> MKLIGIKTSNCFLVSDNIEGKRYFHSQLDELLFDGKRATETYKSDWFKLEKEPSVIEKQMPAKKINHRYELKEGFQESELTPKVIKASYIGEDSEYYEVKGLYDLKFEEIP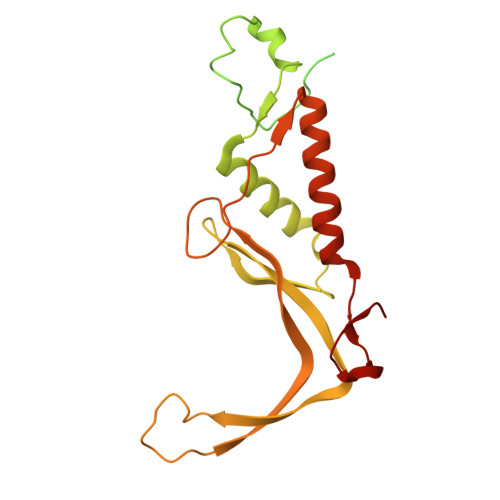QQNEKIEFEMNVIEEIDGELKLQSHNFNLNYNLLDRIQTHPMLLETKPCYLSQEESYKIIRNHIKANINPKFARITSDYDFCLTVVKVLELYKPHEYIVDLNAMYKRRKPKLEKRFQTKREVEIYKVAPKAYQSYPIVEPFSGKDVEDLKSNIKKFLDDLMAKINEPLVECKCCKGRGVILNEN> MAHHHHHHMHEDFPRIDPIRLLDDLKTLRSFGATGPGVVRLSLSPVDIDARRWLAGRMTDAGLDAAIDGVGTVFGRSRKPGPALVIGSHSDTQPTGGWLDGALGVIYGLEIARALGECEATREFAVDVASWIDEEGTFSSFLGSRSFVGDAIDDSLRSARNHEG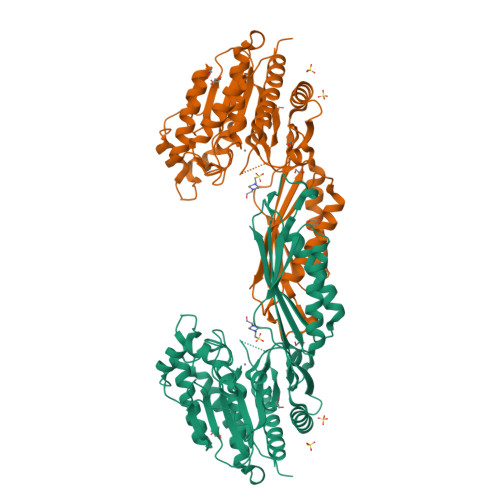LLLGDALAQAGLANTPRVTLDRKRQRAYLEPHIEQGGRLEASAKLIGVVTTIVGIREFQLRFIGQRNHAGTTPMAIRRDAGAALVAFIAHIDDAFGRLADADTVWTVGRIDLDPGSFSVVPGKAVLHLQFRDANPNRLHAMENALVALVDEWNGQHLVRAELIACEGAEEPVTMDAALQQHLAQAADALAPGQWMHMPSGASHDAQVIAQHIPACMLFVPSIGGVSHDFIEDTAEQHIVLGCEVAARAAARIAGALRR Manganese peroxidases (MnPs) are, together with lignin peroxidases and versatile peroxidases, key elements of the enzymatic machineries secreted by white-rot fungi to degrade lignin, thus providing access to cellulose and hemicellulose in plant cell walls. The primary mechanism involves the MnP oxidation of Mn2+ to Mn3+ and the subsequent formation of chelates with fungal dicarboxylic acids. The molecular structures of Ape-MnP1 and Cst-MnP1, which share 50% amino acid sequence identity, are characteristic of ligninolytic peroxidases.

Besides the amino acids of the polypeptide sequences, final models, crystallized in the presence of manganese, contain a heme prosthetic group, two structural calcium ions, and a substrate Mn2+ ion, as well as 180 (Ape-MnP1) and 171 (Cst-MnP1) solvent molecules (with three Mg2+ ions from the crystallization medium also present in the Cst-MnP1 structure). Mn2+ binding was confirmed by anomalous difference electron density maps. Mn2+ oxidation site in Cst-MnP1 also maintains the typical octahedral geometry of the other MnPs. However, this enzyme features only two amino acids (Glu36 and Asp176) as Mn2+ ligands together with three water molecules and the internal heme propionate. Ser40, which occupies the position of the second glutamate acting as a Mn2+ ligand in known long and short MnPs (Glu39 in Pch-MnP1), shows an increase in the Mn-residue bond length to 3.93 Å. This distance leaves Ser40 outside of the coordination sphere in Cst-MnP1, confirming that this residue is not involved in Mn2+ binding. As for Cst-MnP1, the E36A substitution in the Cst-MnP1-E36A variant resulted in the complete loss of the enzyme's ability to oxidize Mn2+, as expected given that Glu36 is one of the only two amino-acid residues (along with Asp176) that contribute to Mn2+ coordination in this enzyme. Regarding Cst-MnP1, the analysis of the E36A variant demonstrated that a single acidic residue (Asp176) at the Mn2+ oxidation site is insufficient for the catalytic process, as previously observed in a VP mutated variant containing only an Asp at this site. This confirms that the catalytic site of Cst-MnP1, formed by Glu36 and Asp176, fufills the minimum requirements for Cst-MnP1 to act as a MnP. Moreover, this site is stabilized by Ser40, which contributes to anchor the internal heme propionate to the alpha-helix, where Glu36 is located, as inferred from the analysis of the S40A variant.

> VTCPDGHVTANRACCALFPVVQNLQENLFDGGECGEEAHSALRLSFHDAIGFSLNSNKGGGADGSILLFNATELTFHANGGIDDITSRQFPVFETTGLTPGDFVHLAGAVGTANCPGAPRLQFMFGRPPPIAPAPDLTVPEPTDDVDAILARFADAGFDASEVVALLSSHTIAAADVVDVTIPGTPFDSTVGTFDTQVFLEVLLAGRSFPGNGSQPGEVLSPLAGEMRLQSDFVVSRDSRTACLWQAMVNNQQLMVSSFAAAMAKLQVLGQNVNTMVDCSDVIPEPAPFAGPIKFPASFSMADVEQACASTFPQIQTVAGPAPTVAPVPGS CHOLESTERYL LINOLEATE | C45 H76 O2 | 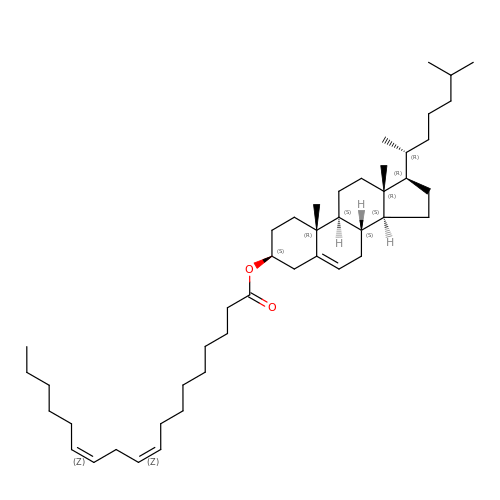NAACPBBQTFFYQB-LJAITQKLSA-N>GAMDEIDDPRIRSVVIVGGGTAGWMTAAALVQHFRTAPLKITVVESSDIGTIGVGEATIPTIRRFYGQLGLRDDDVMRATQATCKLGIRFLDWSGPGSDFIHPFGLYGQDVKGIGFHHYWLKQRRAGDAAPLAAYSLGAALAAGGKFTLPSPHPPSQLSVFDWALHLDAGLFAQHLRAYAEAGGCARIDARIRSVELRPEDGFVRALTLDDGREVEGDLFVDCSGFKGLVIGEALGVGFEDWGRWLPCDAAYAVQSENRPGDAPAPFTRVTARSAGWQWGIPLRHRAGNGLVFSSAHLSDDQALAELMPHLLGDPLTEPRRIPFRPGRRSQAWAKNCVAIGLSSGFLEPLESTSIALIETGIERLKALFPDRRFAQPILDEFNDQTAREMERVRDFIILHYKLNRRTDTDFWRDCREMPVPE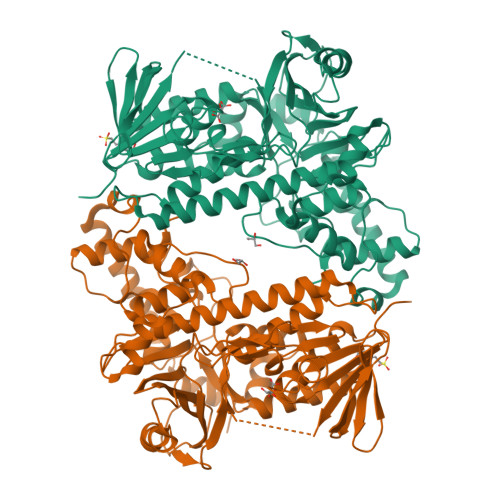TLERKIALWTARGQFVRYRWEMFHPASWLAIYDGFGLYPDHHDPAVDAMDPAYLARSLAEMRANIADLVARTPEHAQFLAGLDPAASAA[2x]(2R,3aR,6R,7S,7aR)-2-[(2S)-2-amino-3-hydroxy-3-oxo-propyl]-6,7-dihydroxy-3,3a,5,6,7,7a-hexahydrofuro[4,5-b]pyran-2-carboxylic 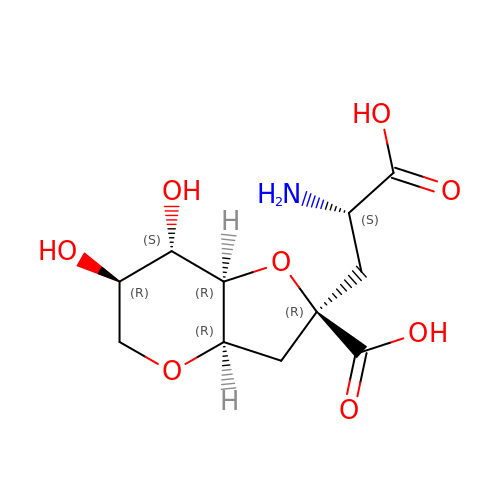acid | C11 H17 N O8 | NRTJEXLNSCGBJU-JROTZIKASA-N> MSGRVGDLSPRQKEALAKFRENVQDVLPALPNPDDYFLLRWLRARSFDLQKSEAMLRKHVEFRKQKDIDNIISWQPPEVIQQYLSGGMCGYDLDGCPVWYDIIGPLDAKGLLFSASKQDLLRTKMRECELLLQECAHQTTKLGRKVETITIIYDCEGLGLKHLWKPAVEAYGEFLCMFEENYPETLKRLFVVKAPKLFPV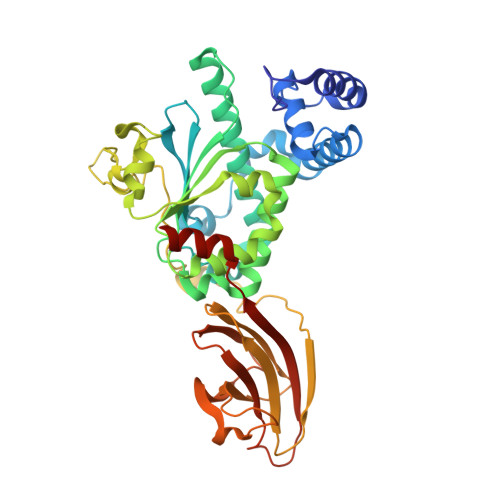AYNLIKPFLSEDTRKKIMVLGANWKEVLLKHISPDQVPVEYGGTMTDPDGNPKCKSKINYGGDIPRKYYVRDQVKQQYEHSVQISRGSSHQVEYEILFPGCVLRWQFMSDGADVGFGIFLKKKMGERQRAGEMTEVLPNQRYNSHLVPEDGTLTCSDPGIYVLRFDNTYSFIHAKKVNFTVEVLLPDKASEEKMKQLGAGTPK>[2x]MINVSDLT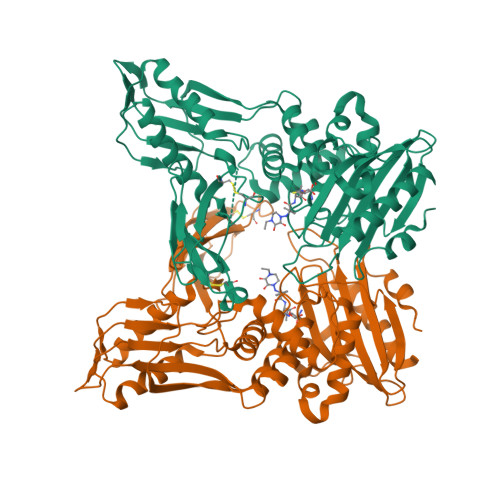QKLPEGSNAGVIAKNINQNQIIADYNGSTFMLPASTQKVFTAVAAKLALGDQFQFETALLSNGKIQNGNLDGNLIVSFTGDPDLTRGQLYSLLAELKKQGIKKINGDLVLDTSVFSSHDRGLGWIWNDLTMCFNSPPAAANIDNNCFYAELDANKNPGEIVKINVPAQFPIQVFGQVYVADSNEAPYCQLDVVVHDNNRYQVKGCLARQYKPFGLSFAVQNTDAYAAAIIQRQLRKLGIEFNGKVLLPQKPQQGQLLAKHLSKPLPDLLKKMMKKSDNQIADSLFRAVAFNYYKRPASFQLGTLAVKSILQKQGIRFGNSILADGSGLSRHNLVAPKTMLSVLEYIAKNEDKLHLMETFPIAGVDGTISGRGGLISPPLVKNVIAKTGSLKGVYNLAGFMTNARGEKVAFVQFINGYSTGDLESKTKRAPLVQFERNLYNELYKY> MDYKDDDDKGDYKDDDDKIDYKDDDDKGSMEEISTDPVVPAVKPDPRTSSVGEGANRHENDDGGSGGSEIGAPDL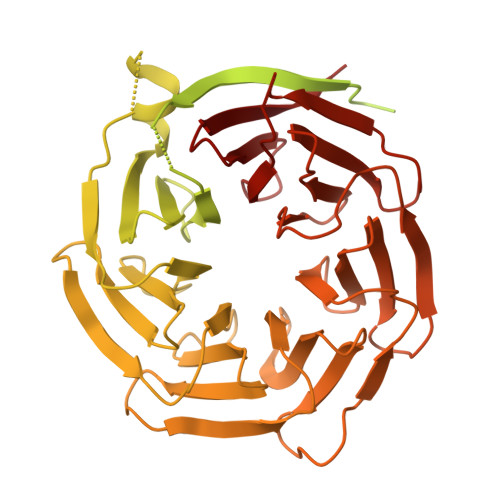DKDLLCPICMQIIKDAFLTACGHSFCYMCIITHLRNKSDCPCCSQHLTNNQLYPNFLLDKLLKKTSARHVSKTASPLDQFREALQRGCDVSIKEVDNLLTLLAERKRKMEQEEAERNMQILLDFLHCLRKQKVDELNEVQTDLQYIKEDINAVERHRIDLYRARDRYSVKLRMLGDDPSTRNAWPHEKNQIGFNSNSLSIRGGNFVGNYQNKKVEGKAQGSSHGLPKKDALSGSDSQSLNQSTVSMARKKRIHAQFNDLQECYLQKRRQLADQPNSKQENDKSVVRREGYSNGLADFQSVLTTFTRYSRLRVIAEIRHGDIFHSANIVSSIEFDRDDELFATAGVSRCIKVFDFSSVVNEPADMQCPIVEMSTRSKLSCLSWNKHEKNHIASSDYEGIVTVWDVTTRQSLMEYEEHEKRAWSVDFSRTEPSMLVSGSDDCKVKVWCTRQEASVINIDMKANICCVKYNPGSSNYIAVGSADHHIHYYDLRNISQPLHVFSGHKKAVSYVKFLSNNELASASTDSTLRLWDVKDNLPVRTFRGHTNEKNFVGLTVNSEYLACGSETNEVYVYHKEITRPVTSHRFGSPDMDDAEEEAGSYFISAVCWKSDSPTMLTANSQGTIKVLVLAA[(1R,3R,4R,7S)-7-HYDROXY-3-(GUANIN-9-YL)-2,5-DIOXABICYCLO[2.2.1]HEPT-1-YL]METHYL DIHYDROGEN PHOSPHATE | C11 H14 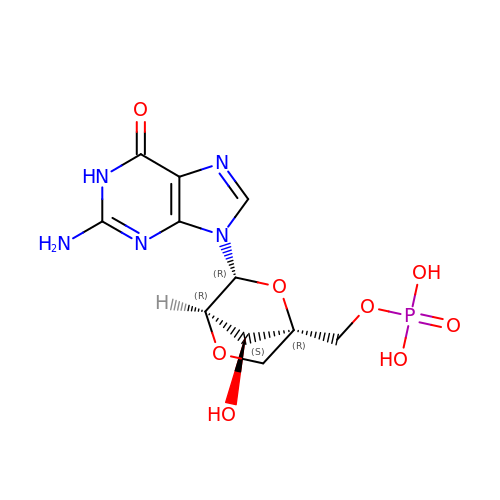N5 O8 P | FZGXOAHULCKQGE-HLJYALQUSA-N The injectisome is a specialized bacterial organelle that utilizes a type III secretion system (T3SS) to translocate effector proteins from the bacterial cytosol directly into a eukaryotic host. Composed of >20 different proteins, the injectisome forms a syringe shaped nanomachine that spans both bacterial membranes and that of the infected host. The major structural unit of the injectisome is the basal body, composed of three highly oligomerized concentric rings spanning the bacterial inner membrane (IM) (PrgH and PrgK in the Salmonella enterica serovar Typhimurium SPI-1 T3SS)3–6 and outer membrane (OM)7 (InvG, a member of the secretin family of OM pores also found in the type II secretion system, type IV pili system, as well as the phage assembly system). To address this and further elucidate the structural basis for injectisome assembly and function, including that of the central needle component, we have conducted here a cryo-EM analysis of the assembled native needle complex resulting in 3D reconstructions of the IM and OM rings at resolutions permitting atomic model building (3.6 Å and 3.9 Å, respectively) and the 3D reconstruction of an isolated helical needle filament at 3.3 Å resolution.

The density in the core region (InvG176–557) showed defined secondary structure with the majority of side chains clearly visible allowing for unambiguous building and refinement of the structure including significant additionally resolved and structurally changed regions from the previously determined closed form. The most dramatic conformational change upon needle assembly is in the inner β-barrel. In the fully open state defined here, the GATE1 hairpin is now unkinked, with the residues at the tip having moved position by a remarkable ~40 Å (measured from the Gly395 Cα). The open position is stabilized by intimate packing against the outer β-barrel of itself and neighboring monomer i + 1 (monomers defined clockwise looking down from the OM), and extending vertically toward the lip region of monomer i + 2 with a dramatic increase in buried surface area between the inner and outer β-barrels (2111 Å2 per monomer compared to 1153 Å2 in the closed state). The inner β-barrel strands 6 and 7 (termed GATE2 here) are straightened around Gly430 and Gly451 compared to the closed form. More significantly, the GATE2 loop (residues Asp433-Gly451) undergoes a 180° rotation, effectively repositioning the regions oriented above the GATE1 hairpin in the closed state against the outer β-barrel in the open state. These changes in GATE1 and GATE2 of the inner β-barrel result in an increase in the secretin pore diameter from ~15 Å in the closed state to a remarkable ~75 Å in the open state.

>[15x]MKTHILLARVLACAALVLVTPGYSSEKIPVTGSGFVAKDDSLRTFFDAMALQLKEPVIVSKMAARKKITGNFEFHDPNALLEKLSLQLGLIWYFDGQAIYIYDASEMRNAVVSLRNVSLNEFNNFLKRSGLYNKNYPLRGDNRKGTFYVSGPPVYVDMVVNAATMMDKQNDGIELGRQKIGVMRLNNTFVGDRTYNLRDQKMVIPGIATAIERLLQGEEQPLGNIVSSEPPAMPAFSANGEKGKAANYAGGMSLQEALKQNAAAGNIKIVAYPDTNSLLVKGTAEQVHFIEMLVKALDVAKRHVELSLWIVDLNKSDLERLGTSWSGSITIGDKLGVSLNQSSISTLDGSRFIAAVNALEEKKQATVVSRPVLLTQENVPAIFDNNRTFYTKLIGERNVALEHVTYGTMIRVLPRFSADGQIEMSLDIEDGNDKTPQSDTTTSVDALPEVGRTLISTIARVPHGKSLLVGGYTRDANTDTVQSIPFLGKLPLIGSLFRYSSKNKSNVVRVFMIEPKEIVDPLTPDASESVNNILKQSGAWSGDDKLQKWVRVYLDRGQEAIK>[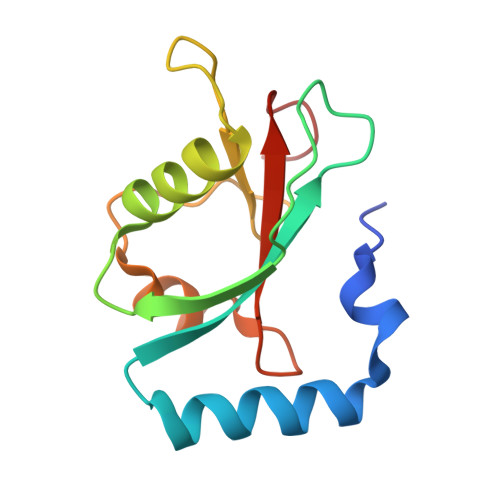2x]GAMSMKWMFKEDHSLEHRCVESAKIRAKYPDRVPVIVEKVSGSQIVDIDKRKYLVPSDITVAQFMWIIRKRIQLPSEKAIFLFVDKTVPQSSLTMGQLYEKEKDEDGFLYVAYSGENTFGF The crystal structures of the niacin-responsive repressor, BhNiaR, which negatively regulates the expression of genes involved in the NAD+ synthesis pathway, were determined to be the apo and niacin-bound forms. Each BhNiaR structure was composed of two domains, an N-terminal DNA-binding domain (residues 1–70) and a C-terminal dimerization/substrate-binding 3H domain (residues 71–179), connected by a flexible loop (residues 66–75). Three highly conserved histidines (His83, His150, and His152) and a glutamate (Glu91) form a binding site for the zinc ion and niacin. BhNiaR formed a dimer between the C-terminal domains as well as between the N-terminal domain of one subunit and the C-terminal domain of the other subunit, whereas TmNiaR formed a dimer through the C-terminal domains alone.

The apo crystal structure of BhNiaR was refined to 2.0 Å resolution with crystallographic Rwork and Rfree values of 20.18% and 22.78%, respectively. Although the refined model contained a subunit in an asymmetric unit composed of 173 residues with a zinc ion and 129 water molecules, it could be generated to a homo-dimeric structure by a symmetric subunit. The N-terminal region (residues 1–6), the linker loop region (residues 68–74) connecting the N- and C-terminal domains, and the internal region (residues 137–147) in the C-terminal domain were poorly ordered due to lack of electron-density maps. However, in the apo structure of BhNiaR, three residues (Glu91, His150, and His152), corresponding to TmNiaR residues (Glu87, His146, and His148), and a water molecule coordinated with a zinc ion in tetrahedral geometry: Glu91 Oε1, His150 Nε1, His152 Nε2, and Wat108 O. The His83 residue was not involved directly in metal coordination, with a distance of 3.8 Å. The zinc ion is located between layered α-helices and a β-sheet of the C-terminal domain. A dimeric BhNiaR structure was generated by a crystallographic twofold symmetry. It seems that both the apo and niacin-bound BhNiaR structures display non-DNA bound conformations because of the crystal packing and interactions between the N- and C-terminal domains of each subunit in the dimer.

> MSDEKKILGEERRSLLIKWLKASDTPLTGAELAKRTNVSRQVIVQDVSLLKAKNHPILATAQGYIYMKEANTVQAQRVVACQHGPADMKDELLTLVDHGVLIKDVTVDHPVYGDITASLHLKSRKDVALFCKRMEESNGTLLSTLTKGVHMHTLEAESEAILDEAIRALEEKGYLLNSF> MSLSNKLTLDKLDVKGKRVVMRVDFNVPMKNNQITNNQRIKAAVPSIKFCLDNGAKSVVLMSHLGRPDGVPMPDKYSLEPVAVELKSLLGKDVLFLKDCVGPEVEKACANPAAGSVILLENLRFHVEEEGKAKDASGNKVKAEPAKIEAFRASLSKLGDVYVNDAFGTAHRAHSSMVGVNLPQKAGGFLMKKELNYFAKALESPERPFLAILGGAKVADKIQLINNMLDKVNEMIIGGGMAFTFLKVLNNMEIGTSLFDEEGAKIVKDLMSKAEKNGVKIT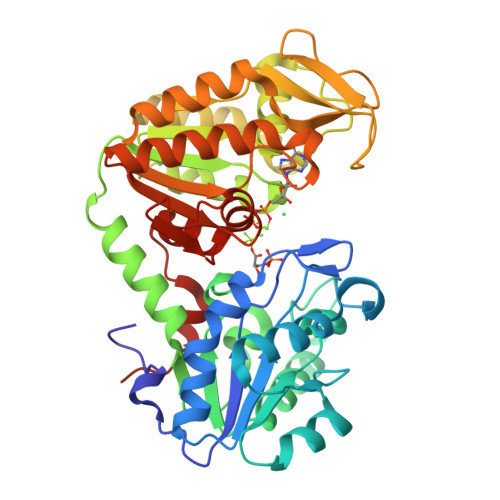LPVDFVTADKFDENAKTGQATVASGIPAGWMGLDCGPESSKKYAEAVTRAKQIVWNGPVGVFEWEAFARGTKALMDEVVKATSRGCITIIGGGDTATCCAKWNTEDKVSHVSTGGGASLELLEGKVLPGVDALSNI> MVPDWEEVLGLWRAGRYYEVHEVLEPYWLKATGEERRLLQGVILLAAALHQRRLGRPGLRNLRKAEARLEGLPCPLM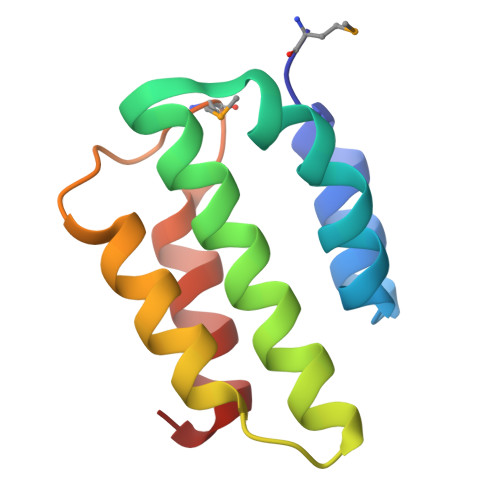GLDWRSLLQEARRRLGA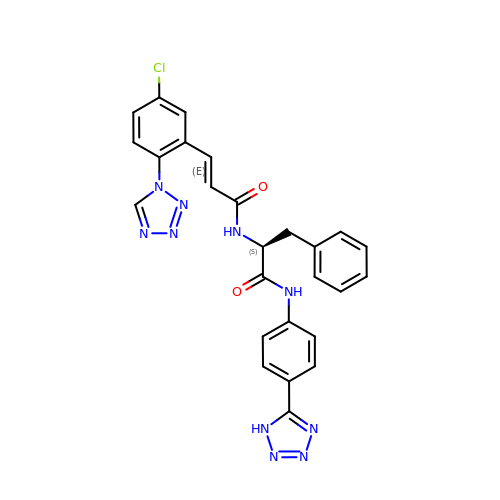(2S)-2-[[(E)-3-[5-chloranyl-2-(1,2,3,4-tetrazol-1-yl)phenyl]prop-2-enoyl]amino]-3-phenyl-N-[4-(1H-1,2,3,4-tetrazol-5-yl)phenyl]propanamide | C26 H21 Cl N10 O2 | YGQQLNQKNAXOKN-SYZXBLONSA-N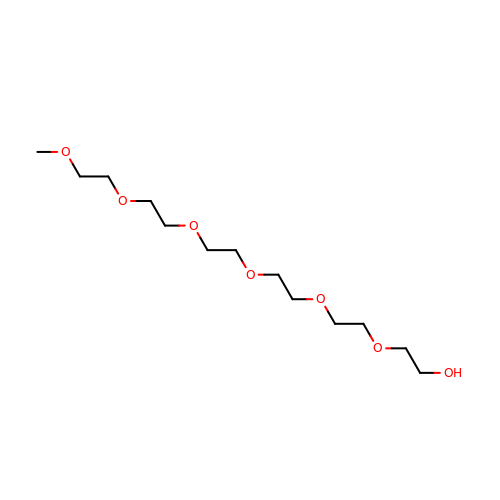2,5,8,11,14,17-HEXAOXANONADECAN-19-OL | C13 H28 O7 | FHHGCKHKTAJLOM-UHFFFAOYSA-N>[2x]MDTPRPQLLDFQFHQNNDSFTLHFQQRLILTHSKDNPCLWIGSGIADIDMFRGNFSIKDKLQEKIALTDAIVSQSPDGWLIHFSRGSDISATLNISADDQGRLLLELQNDNLNHNRIWLRLAAQPEDHIYGCGEQFSYFDLRGKPFPLWTSEQGVGRNKQTYVTWQADCKENAGGDYYWTFFPQPTFVSTQKYYCHVDNSCYMNFDFSAPEYHELALWEDKATLRFECADTYISLLEKLTALLGRQPELPDWIYDGVTLGIQGGTEVCQKKLDTMRNAGVKVNGIWAQDWSGIRMTSFGKRVMWNWKWNSENYPQLDSRIKQWNQEGVQFLAYINPYVASDKDLCEEAAQHGYLAKDASGGDYLVEFGEFYGGVVDLTNPEAYAWFKEVIKKNMIELGCGGWMADFGEYLPTDTYLHNGVSAEIMHNAWPA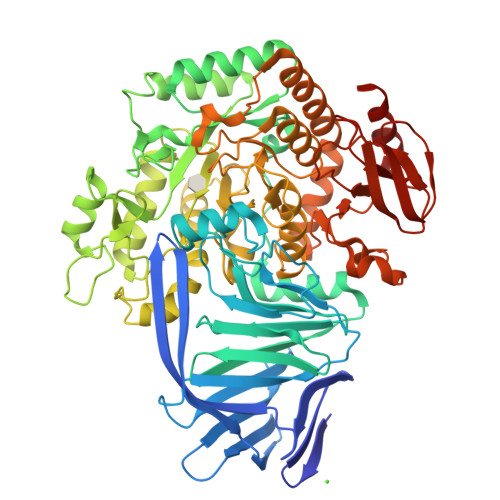LWAKCNYEALEETGKLGEILFFMRAGSTGSQKYSTMMWAGNQNVDWSLDDGLASVVPAALSLAMTGHGLHHSDIGGYTTLFEMKRSKELLLRWCDFSAFTPMMRTHEGNRPGDNWQFDGDAETIAHFARMTTVFTTLKPYLKEAVALNAKSGLPVMRPLFLHYEDDAHTYTLKYQYLLGRDILVAPVHEEGRSDWTLYLPEDNWVHAWTGEAFRGGEVTVNAPIGKPPVFYRADSEWAALFASLKSILEHHHHHH> MSKRKFKEELLEALVPEIYGPAADVKPDIKPRALKRVKK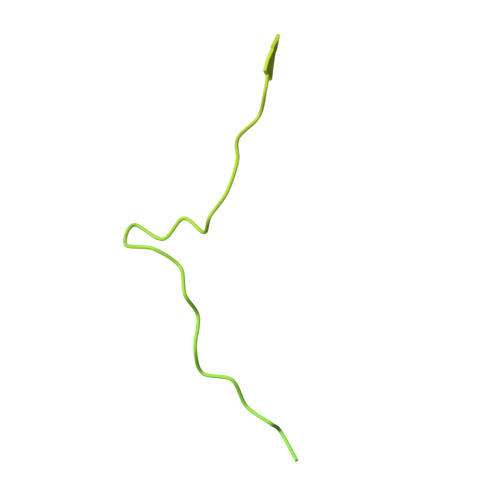REKKEETGLLDDDVEFVRTFAPRRQVQWRGRKVKRVLRPGTTVVFTPGERSATRALKREYDEVYADEDILEQAAQQIGEFAYGKRGRYGEVGLLLDQSNPTPSLKPATQQQILPVTETKRGVKRENKDELQPTMQLMVPKRQKLEEVLENMKVDPSVEPEVKVRPIKEIGPGLGVQTVDIQIPVRTTPAVAMAEAMETQTDQPAAVTTREIGLQTDPRYESVTSTRRSRGRKYTAANSILPEYALHPSITPTPGYRGTIFRPSRPRTTRRRRTTRRRSRRITPISVHRVTRRGRTITLPNARYHPSILI>[2x]MKPKVFITREIPEVGIKMLEDEFEVEVWGDEKEIPREILLKKVKEVDALVTMLSERIDKEVFENAPKL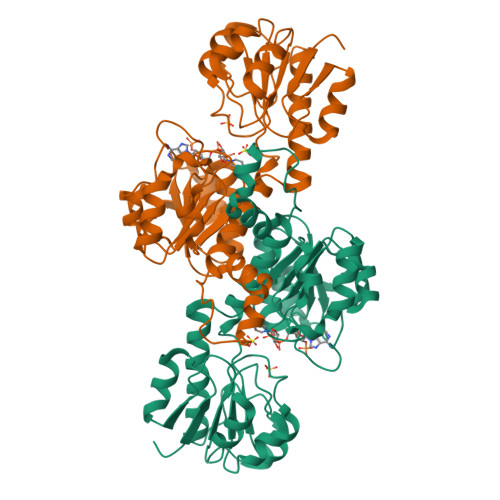RIVANYAVGYDNIDIEEATKRGIYVTNTPDVLTDATADLAFALLLATARHVVKGDRFVRSGEWKKRGVAWHPKWFLGYDVYGKTIGIIGLGRIGQAIAKRAKGFNMRILYYSRTRKEEVERELNAEFKPLEDLLRESDFVVLAVPLTRETYHLINEERLKLMKKTAILINIARGKVVDTNALVKALKEGWIAGAGLDVFEEEPYYNEELFKLDNVVLTPHIGSASFGAREGMAELVAKNLIAFKRGEIPPTLVNREVIKIRKPGFE>[2x]SGISLDNSYKMDYPEMGLCIIINNKNFHKSTG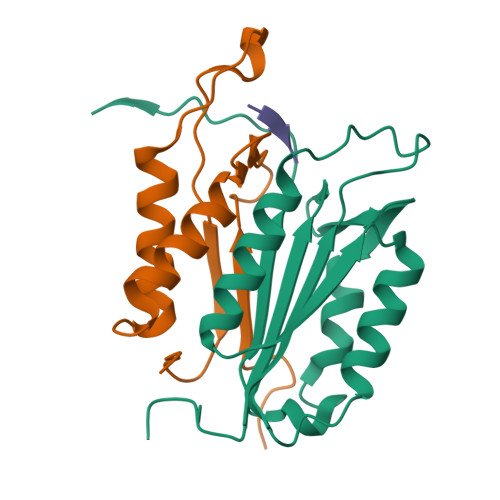MTSRSGTDVDAANLRETFRNLKYEVRNKNDLTREEIVELMRDVSKEDHSKRSSFVCVLLSHGEEGIIFGTNGPVDLKKITNFFRGDRCRSLTGKPKLFIIQACRGTELDCGIETD;>SGVDDDMACHKIPVEADFLYAYSTAPGYYSWRNSKDGSWFIQSLCAMLKQYADKLEFMHILTRVNRKVATEFESFSFDATFHAKKQIPCIVSMLTKELYFYHHHHHHH[2x];>XIEPD[2x]> MAYPGHPGAGGGYYPGGYGGAPGGPAFPGQTQDPLYGYFAAVAGQDGQIDADELQRCLTQSGIAGGYKPFNLETCRLMVSMLDRDMSGTMGFNEFKELWAVLNGWRQHFISFDTDRSGTVDPQELQKALTTMGFRLSPQAVNSIAKRYSTNGKITFDDYIACCVKLRALTDSFRRRDTAQQGVVNFPYDDFIQCVMSV;> MAYPGHPGAGGGYYPGGYGGA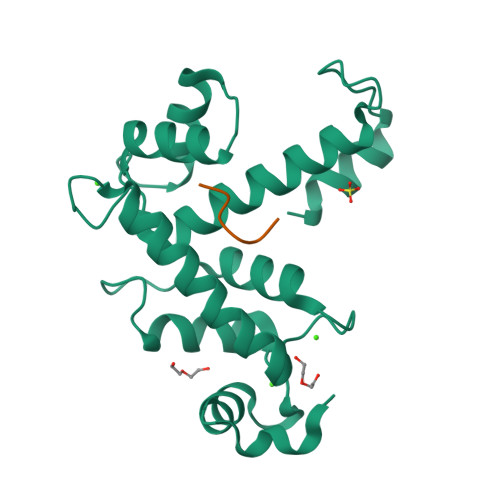PGGPAFPGQTQ>[2x]MPPYTVVYFPVRGRCAALRMLLADQGQSWKEEVVTVETWQEGSLKASCLYGQLPKFQDGDLTLYQSNTILRHLGRTLGLYGKDQQEAALVDMVNDGVEDLR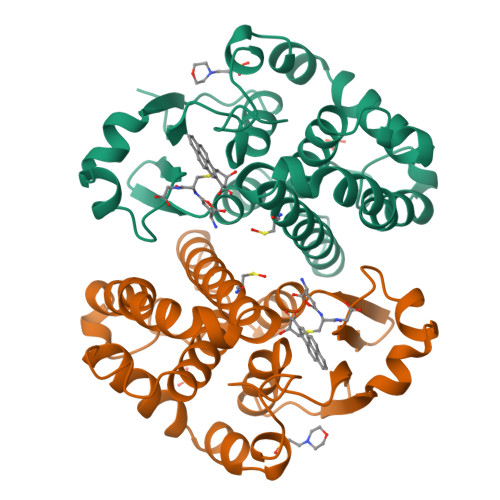CKYVSLIYTNYEAGKDDYVKALPGQLKPFETLLSQNQGGKTFIVGDQISFADYNLLDLLLIHEVLAPGCLDAFPLLSAYVGRLSARPKLKAFLASPEYVNLPINGNGKQ>[2x]GAMPHDPSFTPTQLAARAAYLLRGNDLGTMTTAAPLLYPHMWSWDAAFVAIGLAPLSVERAVVELDTLLSAQWRNGMIPHIVFANGVDGYFPGPARWATATLADNAPRNRLTSGITQPPVHAIAVQRILEHARTRGRSTRAVAEAFLDRRWGDLMRWHRWLAECRDRNERGRITLYHGWESGMANSPRWDSAYANVVPGKLPEYQRADNVIITDPSQRPSDGEYDRYLWLLEEMKAVRYDDERLPSVMSFQVEDVFFSAIFSVACQVLAEIGEDYKRPHADVKDLYLWAERFRAGVVETTDQRTGAARDFDVLAEKWLVTETAAQFAPLLCGGLPHDRERALLKLLEGPRFCGHPDLKYGLIPSTSPVSRDFRPREYWRGPVWPVLTWLFSWCFARRGWAERARLLRQEGLRQASDGSFAEYYEPFTGEPLGSMQQSWTAAAVLDWLG

A glucosylglycerate hydrolase (GgH) identified in M. hassiacum and found to be highly conserved among rapidly growing mycobacteria is likely to be responsible for the rapid mobilization of GG accumulated during nitrogen starvation by hydrolysing it to glucose and glycerate. The MhGgH monomer displays an (α/α)6-barrel domain typical of glycoside hydrolase family 63 (GH63), to which MhGgH belongs. While the active site of GH63 members acting on larger substrates is located in an open, solvent-accessible cleft, those of MhGgH and of MgH from T. thermophilus are covered by a cap domain (subdivided into A′- and B′-regions) with constrained access through a narrow negatively charged tunnel. The crystallographic structure of MhGgH revealed a homotetrameric architecture, which is compatible with the oligomeric organization of the enzyme in solution as assessed by SAXS.

MhGgH was unable to hydrolyse GGlycerol and GGlycolate, despite their considerable similarity to GG. The structures of the E419A variant in complex with both compounds and that of the D182A variant in complex with GGlycolate were determined and help in understanding this behaviour. The most significant differences from the complexes with GG/MG are observed at subsite +1. In the case of GGlycolate, the glycolate moiety is found in a single position in the E419A variant but adopts two different conformations in the D182A variant. In the D182A variant, one of the glycolate conformations is close to that found in the E419A variant (direct contacts with Trp40 and Tyr88 and water-mediated interactions with Gln115 and Trp177), while the second conformation of the ligand is stabilized by hydrogen bonds to Tyr88, Arg216 and Tyr375 and by solvent-mediated contacts with Phe89, Trp177 and Tyr222. In particular, interactions with Tyr36, a key residue for active-site closure and organization, are always absent, while different subsets of interactions are observed for GGlycerol and GGlycolate. Any deviation from these strict interaction patterns will result in a decreased affinity for and highly reduced activity towards the compound, as observed for GGlycerol and GGlycolate.2-[4,6-dimethyl-3-(1H-pyrrol-1-yl)-1H-pyrazolo[3,4-b]pyridin-1-yl]-N-[3-(morpholin-4-yl)propyl]acetamide 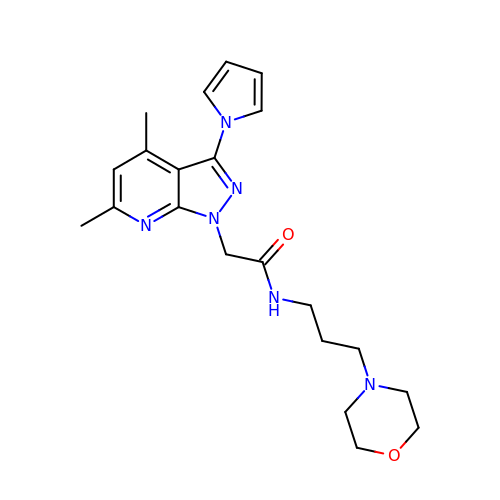| C21 H28 N6 O2 | AZMBNAXBTVHIKQ-UHFFFAOYSA-N> HHHHHHKWLGGKTTNENAAYYQVVPVTANVYDSDGEKLSYISQGSVVWLDKDRKSDDKRLAITISGLSGYMKTEDLQALDASKDFIPYYESDGHRFYHYVAQNASIPVASHLSDMEVGKKYYSADGLHFDGFKLENPFLFKDLTEATNYSAEELD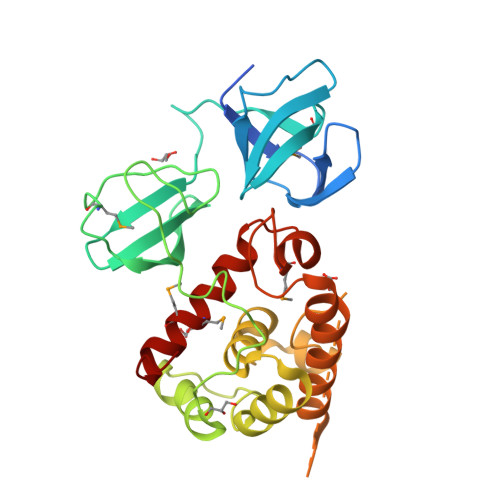KVFSLLNINNSLLENKGATFKEAEEHYHINALYLLAHSALESNWGRSKIAKDKNNFFGITAYDTTPYLSAKTFDDVDKGILGATKWIKENYIDRGRTFLGNKASGMNVEYASDPYWGEKIASVMMKINEKLGGKD NarK is highly expressed during anaerobic growth in the presence of nitrate, and plays a central role in nitrate uptake, while NarU has important functions during severe nutrient starvation or slow growth. In this work, we demonstrate that NarK is a nitrate/nitrite antiporter, using an in vitro reconstituted system. The overall structures of NarK in both the occluded and inward-open states adopt a canonical MFS-fold with 12 TM helices, with TM1–TM6 and TM7–TM12 forming the N and C bundles, respectively. The substrate-binding site is located at the interface between the N and C bundles, in the middle of the TM segment.

Each asymmetric unit of Crystals I and II contained one inward-open molecule, while in the asymmetric unit of Crystal III, there were two occluded molecules (Mol A and B). In the nitrate-bound occluded structure, we observed a strong electron-density peak in the substrate-binding site. The crystallization conditions for the occluded-state crystals (Crystal III) contained ammonium nitrate. Therefore, we assigned this peak as a nitrate ion. The nitrate ion is sandwiched between F147 and F267, and forms a π–π stacking interaction with the π electrons of their phenyl groups. In Site A, two oxygen atoms of the nitrate ion form a bidentate salt bridge with the NH1 and NH2 atoms of the R89 guanidinium group. In Site B, two oxygen atoms of the nitrate ion form a bifurcated hydrogen bond with the phenol hydroxyl group of Y263 in TM7. In layer C3, part of the N-terminal loop consisting of P20 and E21 forms van der Waals contacts with the cytosolic terminus of TM11, including D392, E393 and M396. These interactions between the N and C bundles tightly close the pathway to the cytoplasmic side to prevent the intrusion of water or other solvent molecules into the substrate-binding site. In each of three independent simulations starting from the occluded state with the bound nitrate, no large structural change in the overall conformation was observed during the 250-ns simulation, suggesting that the overall structure of the occluded state is stable in the lipid bilayer environment. In the nitrate-bound occluded state, the negative charge of the nitrate in the substrate-binding site relaxes the electrostatic repulsion between the two positively charged arginine residues (R89 and R305), thereby enabling these two arginine residues to be in close proximity in the low-dielectric intramembrane environment.

>[2x]MSHSSAPERATGAVITDWRPEDPAFWQQRGQRIASRNLWISVPCLLLAFCVWMLFSAVAVNLPKVGFNFTTDQLFMLTALPSVSGALLRVPYSFMVPIFGGRRWTAFSTGILIIPCVWLGFAVQDTSTPYSVFIIISLLCGFAGANFASSMANISFFFPKQKQGGALGLNGGLGNMGVSVMQLVAPLVVSLSIFAVFGSQGVKQPDGTELYLANASWIWVPFLAIFTIAAWFGMNDLATSKASIKEQLPVLKRGHLWIMSLLYLATFGSFIGFSAGFAMLSKTQFPDVQILQYAFFGPFIGALARSAGGALSDRLGGTRVTLVNFILMAIFSGLLFLTLPTDGQGGSFMAFFAVFLALFLTAGLGSGSTFQMISVIFRKLTMDRVKAEGGSDERAMREAATDTAAALGFISAIGAIGGFFIPKAFGSSLALTGSPVGAMKVFLIFYIACVVITWAVYGRHSKKLESSGENLYFQG>GSHMTGPVTKEDLGRATWTFLHTLAAQYPEKPTRQQKKDVKELMTILSRMYPCRECAD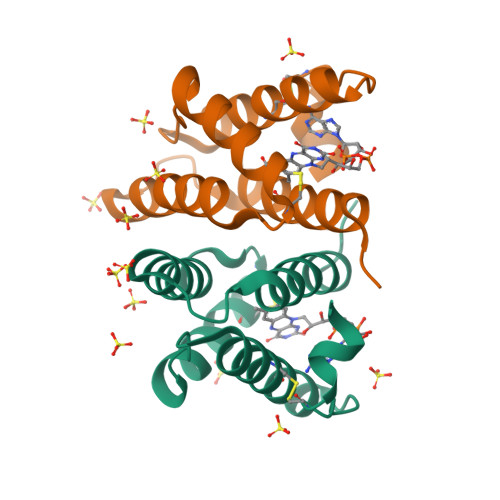HFKEILRSNPAQAGSQEEFSQWLCHVHNTVNRSLGKLVFPCERVDARWGKLECEQKSCDLHGTSMDF[2x]2-(4-methylpiperazin-1-yl)-1,3-benzothiazole | C12 H15 N3 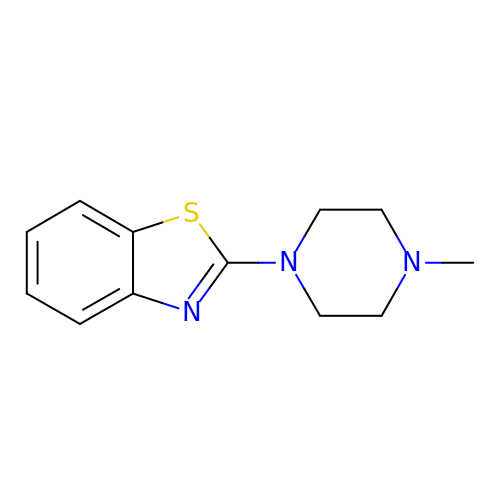S | DZERTEQKWVKWJP-UHFFFAOYSA-N> YPFVEP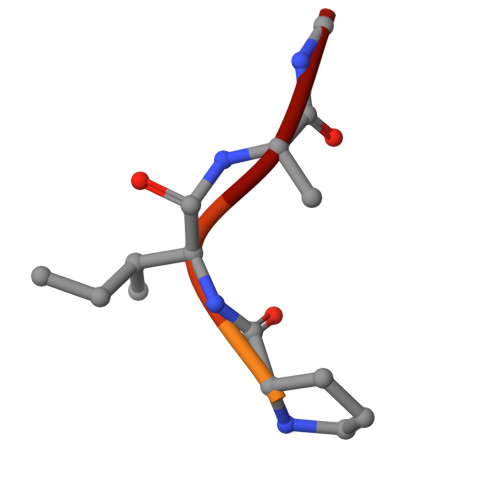IDF2-[[6,7-bis(chloranyl)-2-cyclopentyl-2-methyl-1-oxidanylidene-3~{H}-inden-5-yl]oxy]ethanoic acid | C17 H18 Cl2 O4 | 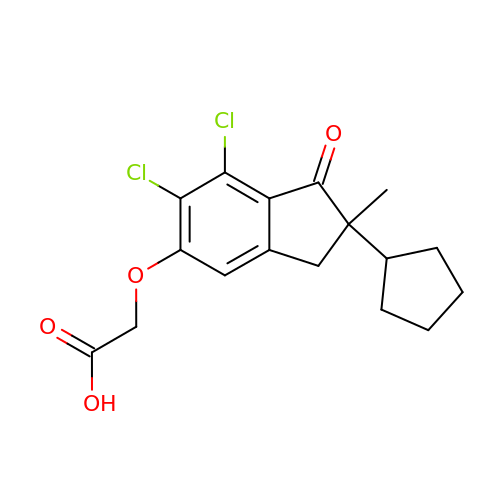RNOJGTHBMJBOSP-UHFFFAOYSA-N> MHHHHHHASGLVPRGSHMTRTTALKVLAGKKLTDLDPAEWAKAQASAERILVDVGTGDARTAYRQAIAHPEWLVVGVDPAWQRMTETAVRAARKPAKGGAPNLVLVSSAIETVPAALHGVADEVMVLMPWGKLLRGVVLGEADVLSGLRAVAKPGAPLEISIGTSIWREPIPLEIRDLPELTPETVVSTGLTDRLAALGWQVADVRLVPHTDLDTISSSW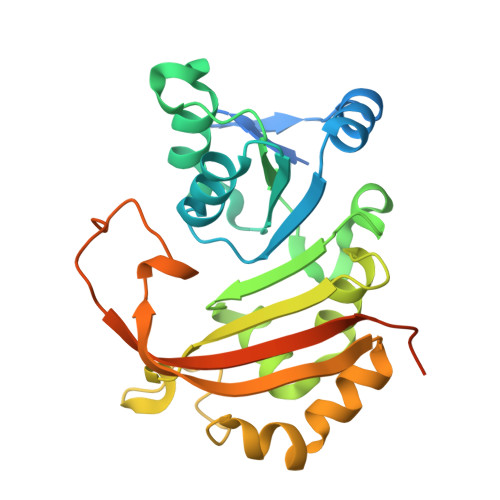ARRLGSGATETVLHLRAVAVDPRDPVGTQHPAAESAQDTPEEPQRDV> MFNRITASSSKEYLPDLLLFWQNYEYWITNIGLYKTKQRDLTRTPANLDTDTEECMFWMNYLQKDQSFQLMNFAMENLGALYFGSIGDISELYLRVEQYWDRRADKNHSVDGKYWDALIWSVFTMCIYYMPVEKLAEIFSVYPLHEYLGSNKRLNWEDGMQLVMCQNFARCSLFQLKQCDFMAHPDIRLVQAYLILATTTFPYDEPLLANSLLTQCIHTFKNFHVDDFRPLLNDDPVESIAKVTLGRIFYRLCGCDYLQSGPRKPIALHTEVSSLLQHAAYLQDLPNVDVYREENSTEVLYWKIISLDRDLDQYLNKSSKPPLKTLDAIRRELDIFQYKVDSLEED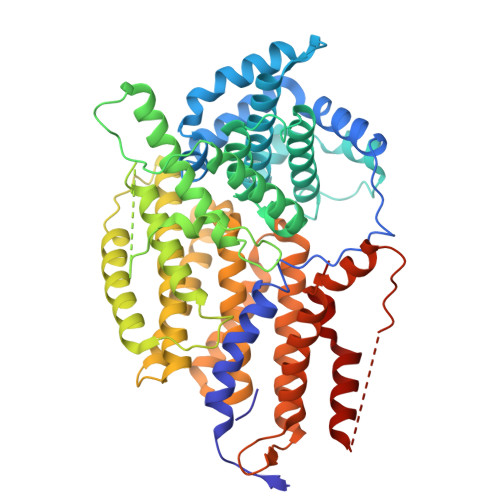FRSNNSRFQKFIALFQISTVSWKLFKMYLIYYDTADSLLKVIHYSKVIISLIVNNFHAKSEFFNRHPMVMQTITRVVSFISFYQIFVESAAVKQLLVDLTELTANLPTIFGSKLDKLVYLTERLSKLKLLWDKVQLLDSGDSFYHPVFKILQNDIKIIELKNDEMFSLIKGLGSLVPLNKLRQESLLEEEDENNTEPSDFRTIVEEFQSEYNISDILS> MEKFGLKALVPLLKLEDKELSSTYDHSMTLGADLSSMLYSLGIPRDSQDHRVLDTFQSPWAETSRSEVEPRFFTPESFTNIPGVLQSTVTPPCFNSIQNDQQRVALFQDETLFFLFYKHPGTVIQELTYLELRKRNWRYHKTLK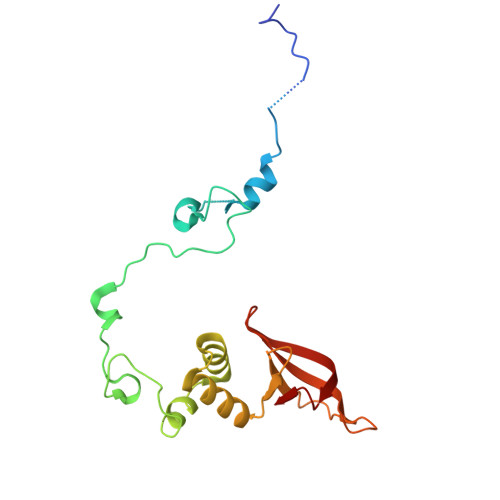AWLTKDPMMEPIVSADGLSERGSYVFFDPQRWEKCQRDFLLFYNAIM> MADGPSPIRIVLWNDGGESLAAGVEDEEQQQVLHSFADLVGSAIDAVLELPQFRHVEAVTAEAEEDEPGLSIGFDAGSGDGEVDIDNLKGRLDIAGLLLGSAQLPEELAEVAAVEVTDEEEGTTELQFTDEGLVQQLQAVVKRAKLEKRYNDWVAGVAESLGPALDAAAGGVEVTEMPVDPYDVLQAVVAQLIRVAGVSPPAPSLFSRTGALVGGVLGAPRSAVRQVTKRLGRAQRLWWRLEDVVVDGSKLALRLAVKAARPVLVGFVLHRVLKTLDRSRQLEYRLARMGPEEAREAYYEAVLGKDWKQQLQADWDKALEDVDAGLVTDEINHEKRLMTAAQLRRLEVEEWDKQRMKNFYLASFGGLRWFDQMEQALHNPLFIESRGWTDPVQNWVGQNRTYMDDLPAGQYMAGVGNAAIRIKEAELKRKLTDVERAHVLARGGAVAGGLLPQQPTDPATLAVAVGGAFVPSVAGKR;> MGASQESELDFVPRLSFLPIEWRSIGSAFGLKDKSGAAANGRATFTVRQGVDAAELTSTGRVIDGQADVGASLKLNTLAIGVSASNITFHSGLDDPTAAAAQRSSLIPSLKLTAAKQFKRDNYIAVSYDLKHQKPELSACWTGEAGADRATLLVNVDPVMRSVKLAAAVRTPGPEWRKVLYNDETDLLEYPADDGARHTLYVQHEVRGRDLLHATRLGCRLDLGRLVNYVVDFVDYRIEENIPSFVWNVPLLPQLYSLLVPADNDEQVRHRITGWELDVSHDFARSGLLPVVAISKTSKKLLGGGTLTASYDAAAREAGVSLSRKGVSVGARVARAEGAAGGLSAGWGRPSIHVAVEPLGLLQ;> MQGLKATPGLRASSGRPTLRTARTALVVRAHASQPSSSNHAEQQECSSSGSGVSVNQPSALGRLGKFGLSSALSAFVLVPNFGGFGGNGGNRGGGGGGGGGGGSGGQGQPDGGLPLPLYELAEESSDEKEKQQKDDKRNWKNLVTDSEDLEEKPGERSGTNRCVEIVIEGWPDVGNLPTADELKDLLTVQEGHIFEKQDLLDDRRKLEIQYEDYIAEVEIRTEYVDGKSNHQRVVYKFTPHQFRGINAIDIKGAALMPASEVERICNECLPKQPYMVDIAVMDKVRNRIEQWYQSRGLPFCYVGFFDGMDDGILRANVTEAKIDNVSVRFVRPKLTGDSELEYSVYDEGKVVKADKIIEASGFQRGHHYHVEDGYDAMNSIFACGLLEDINIEPEQDPSDVNKINVKIRCEEVQPKSMELDLDWSFQLKNGIPSINRQSLIPGGSVEVSHENLFGNSESATLSLSASDWRNPSADLGFSVAYSEPFYKPHTTRNAQLFNTRKTSTIFTPGGESEVPPVFVDRFGLKGWTSQITGQDNKVEHALMLQLVSTLDENGQVVAKGTKVQRGYYADNGPPTTNSGNGRDLSLSYQGFFALDNVRFINGNQLGERMLFQVDQGLNPSISLPGGRKLGLSGGIYNRATASYTKFLEAPFLPKLTTEQLWKERKAPNTVVLHAKAGNALGDVAAYDYFSLGGPYSVRGYSHGEIGAARRFLELATEVRVPLKNYGLPGTAYGFVEYATDLGSGRELNGNPTEYYRKPGRGMSYGLGLKALGACRFEYARDCNAGTGTFLVNFGERF;> MGGGLPPKRSEVAESQPASSASSSAAAPAPAAETAGPKLPPRPAGLGLGGAGLLPSRGAAAAPSAGSATGTPAAAASSSLQQQQQQPAPPATQPAAHAAPAAPAGLGGAGLKPMLPPRPAAAAGAGAAGAAAAKPTPAPAPAAAPVPAAAPPPRPAMPNPAAGMSLPPRPVVAAAPPVLAAAGSDAVVDPSEDRRVQRVQRIAHDTRVRLIRAASRLGLAPRTDQVAQFLQAIERSERMVGAQHYKGSRRVDLLAAAEREARLAEEREGAAAEAVAGLRVKILVLGMTGTGKTELINSLLNRPAGSRTNAFREATRRVRVVRGDHNGIPLTFIDTPGLHASASRTADNRAILRAVRAAYRWHKPDYVFYVDRLDATRPGFGEMGLLGLITESLGAGVWRNTMAVLTHAHAARTAFGGQYDVNSRQRRNIVSQLLRQAAGDQQSRNPVFLADCHPACPTNSLGQPVILEGPTAVPWKQQLLVQLVGYKSYNVATSAFKDLAKAKAGKAAAGAAGGARGPQDIFKQMMRSRLPPMTFFVEQMSEGVLKPEGWATMETVAGLGEEVTEDEGAESFNHVYYRQMYELAVAGDPWAQREYAAMLRAYDKGCESYRASYEEADVDANVEYGVESYVVDPIDFGPSFDPEDMYSHRHAYAEAADAGVTVIPSQDYYGPEHDDPLNGIVFQYEAQPFSRHGWGGVPFDLTVCCEKDKTSLCLQGETHVSLVHSVPPFGPRHITQVTGSWEVLRPNIKDVMYQLEVDTFKDGLLGKSDHAGCGLMLARLGEGGDPRKGPTAVGVRLQDTLRVGPFKLEACASKVAVQGPTGGKEEGWGARAFVGYDWLPGLGMAFDFIQERTPEEGGKRLRGYGANFTYDWEALGAAFGMEVDYVAASESVFVSVNAFSGNDYRLGWLLLLPAVNYFKETVSSLWARLRGAGGGEGEEGEELEEE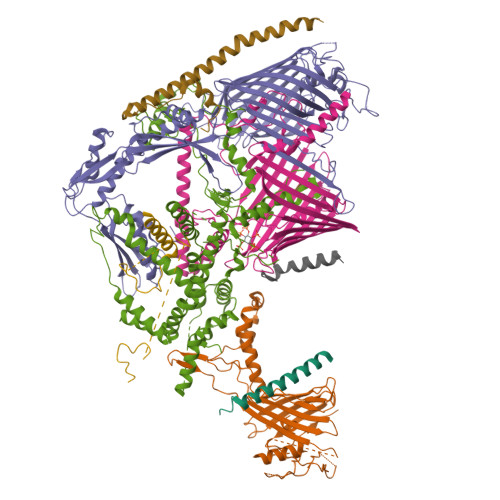GEGEEGDDEEAMMMMAQEGDL;> MITFTFMSLVTSVKDYVEITHKLIEIEPLKNYTEFGAVFTYFIFSIGEFFKNFFSFSFLNNIWSIPIIIPDIASAMISEVSVLDGYFHNAFTFLETSVNTTTNPSLVIFEKFVIGIINSLFLILPTSTSHLITLRRFVMQGLEAGYMAGLGTLAGNFLWLASIILGWRFFVIPWLSLDIFRYLLGFVLLVKYIWDSSKERRMALEDLSKWKIFLLNFLLALTEQSCIYPFISNLSFGPDASILEGFPVDNYPQFLLIHGAYLLGILFGSFSLLQFTCWFWENPAFSIYLWITTKSSLKISTSSYYKILNFTFLYATMLCAIASIPYYGLDYTITNPIGLVPQDRILNQKKSQSDPDKLITETAFLNLNPTDKNSRIRDGVHARRERWKQRLIKYQAFDASTYDQGVYDFLTIEDLNYGFDRFWLRRKMRNHQIRFRLFPGPWMRSLKKQLNNPANPSLETSTKAASGPRVEFFRILFEQFYHPNFHDRAAMQTNPAEARNKFISTSPLASTESKKALNSTFSLGNINNSSTGIEGLVLTNTQATLLPTDLQTKRTIKPGLIYTNSALRKFVRNVNTRLNLKLLNSKETNLTTKYKSQFIYSKRWKSIFSKIQPLQNGTTRKSYQLFRNVAKQILVTPDAKSLKLITINQKLSLKERKLLELRTQYNNNSTLTTTAPLTLVRPLNVYLQKEEAFKRKLRYYGTMPMRKLTVGNQAPYFKALMKRGFYYYKPTLRWRKTLYVASLRRGFRKKSRKQRILVMPSNQQNFNNTLDNTKTNINQNNLANPLGGNEVPMYGADGENSLITKPTHSYTVLGKRASRYRHQIYKDVLQHWYYTPFNRLLMKFDVDAFINRQPKSHFLTKNEERALHIRRFLLSEHYDTLRWYTYMQHYKTMKTNIGGTKSFANRAYNQQFQGTFKKIRHLFAITPKQGDFYTLKFDQPLYNDNKLKDNLYFHEELLTDYYNGTNLQTNQTSNISVNSTTTFIDNSLRTTQLPVPSSSFDIVNQSSTLIGLTTMQNALRKNVVESTLTSLNSDGEAATSQPKLNFVYSELFVKLIKECKKRIHDQTFLKNYITHRIEKREQLNQEQTKELNKRLEKLKVWLNSDKGSISKLQNTPVQDPNISSPDKVLTTAMQKAVNESISLSGIMPSDKIKTTYGNLTNAYTIKTENAILTKLNVINQLTNNETTTQKNTLIKSIGVNKIQTVLQTIITNFKSSLYNQTQLLRVKTDKDLQWWRTKQRVITKRKSARKRDRFKKQIAVVNKKLAALSKKVETEKSNLYQTLYGNYEISDYLLRNVPTGSSAVIDSTVLRKKQDNQAYLPKETNNVQFNSFVDSNNNVWQTFFAKKLRKKISSKGRRYRSLSLARYLTATRKPRLVGLDNLTKIDNITTLQGAFITKEEKQDSLNLTIQRKQELTNSLKKSQIKKRSRHSWKKRSRHQFSRNHYKYRKRHTHGNGKLRVMNKKLKKFKATNELRQWWWNSFLPRYLSNLQVNNSTLTNKNVSFKPLSNTNSVPSTNMASPTTSRNLLDNLNSSNQISTSASMNQNIVTESVKVETNQVYLPEGEKSFDITSMTTTLPFYAGWDESLKKFVVTNRLLSRRDAGLSVNNNPQEINFTNPPIQGLNEGSFLYWQTEMPFNSYNIDQFITTNQSFYAPLGWRRFEFRHSILKTWVNNTKAGNNNIKKKTLIISLKNLQPLKSSQQKQNQIKTKKLVARRIKKRYKLLKQMPNQLMYSPTGPLLTEVLPSHYISVFDQQYRLPRNRYLKRNPLKTLKKTTLLALMDSSKQTNGVNKEFTLRKRVKPRRKYHRKRFIKKDGLIFPRRTKFNTNTTLTGNALITNNVNSIEEDDLRWRPSSRTKQKRKDNTRSSAASKTKSNKRVKTNPLRLRQLRRREFQQVLKPLQRYIPQNGGFTWPGDYLRLEIVEMPKLKSINIKKTSLKQKINVQPVGIMPRKYLIEKHNIKVLKKKLSQAYSTQQLTKVVQEYKNLIQNSPPAI;> MASKKGTDAPAALTDPLKEDPTVIRDEAQFPEPSLYFKVFESEAGEPEAKIRADVNKLYDRWIEKYGRRWPEDGINTEDMVWLAEEANKRKRAKPRPRGTVAAEKTEYEDEFMPDPTVGAPVSAADAAKAARRAKKDRKKKKAAGGAEQPAGPRTNYEKTVAGGKWVTDEFESADYEAGNLEKLWDMYLWDREGKPTMMPDTPAAQQEGEESEDFDDFYTAYRPRDVDSEEAREAVWATDEFESDEDNTESEWAPEYVGAGLGLVAEDPLNPQYSLRHSNHPLAPFPGEPLKWASYVYPDFTTFEGLSKQSIPHGMGVMTFGTGTGAGFAMSQTRYGDKYEGEFQAGYAHGLGQFTSEASGEVYIGEFFAGQRHGCGMTLDMKPYFYLLERGVDPVEAYRRTAGAIMKNVEVRTWYRGNKLGDAKEDEVVEINVLKDELDDPFEIALRNSLHDAKLRKWKAMSPQDKAMDRIVSIIERVQRRNPGRFGAYYREDEKGRVRPVLDSDGADTDFDSVDMIQGVDTDGDLGPGWEGATDSEENPMDPRIRELMAAEGMDDKLEDEGFKDTVLGSAIINPYTGLDMKTYLDGKERHQAELVSVYKASREGRKYLNKVRKDKGGAAKDDESSYVEDDAASGHPGALLSREAEDDRLARLYEQAGVSKEDERRVEGLAARWRRLLAADEEEVLGGAVGAFRRPGNPLAANDSDTGFETESDMMEMCDIPEILGTVQEARQIVERARMWRFKPYGEVGLRMAQDANGSPVSLMQEPLHYPHGTKFMAPGPLGLCHAVPDDPSLRQEMAKVAHNYAAIYRMYNFDWDPEPGTVQYKIDQRIRRAQELRNNAMARYLAAADEVLRDGAAPAGEGDQALLLASTSTGAPEAFDGQGNASGSGSSSALSSRGGSMFASMTLSRPAPMAGVVSLGRAARVVLGAFADAAKSVPMARPRLARPSGRRQ;> MAQPPRPAEEYDDDVQEDEDELKEGELDDDESHEAASEGGEAAAGDEEAEDDEQDEEDGDEDSQPWAGLNRLPERDDMLDILNELRAEGRKQLTVLLLGKSSVGKSSLINSLLGEAVVRVQAFKLQADTDITTTVVRQVAVGNSEVDGFRLKLIDTCGLEDPEAGDTVNLGALSKIAEDVRGVGIDVVLYCDRLDLYRVDPLDKAIIDAISSTFGRGIWRRTVVALTHANLVQTPPGTDYDSFVNGRVRLIRGAVRGPLFFRPSLPVALVENSETCPVSSESGFRVLPDGEPWLVALVSQLVDMAAARRRPYKYHPRLSSKPSHRFRWLLPVAIAAEVLFYRRFLHPRLDDNQRRVEREEERVWALRGQQRRALGLHRPHRPDKDAAWRLEQMYDDD;> AAAAFAFFAGFAFAAFAAAAAAAA>GQDMVSPPPPIADEPLTVNTGIYLIACYSLDDKAETFKVNAFLSLSWKDRRLAFDPVRSGVRVKTYEPEAIWIPEIRFVNVENARDADVVDISVSPDGTVQYLERFSARVLSPLDFRRYPFDSQTLHIYLIVRSVDTRNIVLAVDLEKVGKNDDVFLTGWDIESFTAVVKPANFALEDRLESKLDYQLRISRQYFSYIPNIILPMLFILFISWTAFWSTSYEANVTLVVSTLIAHIAFNILVETNLPKTPYMTYTGAIIFMIYLFYFVAVIEVTVQHYLKVESQPARAASITRASRIAFPVVFLLANIILAFLFFGF[5x]

At present, the best structurally characterized pLGIC is the G. violaceus ligand-gated ion channel (GLIC), of prokaryotic origin. Each subunit consists of an extracellular domain (ECD), predominantly in a β-sandwich fold, and a transmembrane domain (TMD) composed of four helices, labeled M1–M4. However, the GLIC is a pH-gated channel, activated by lowering the pH, with a maximal activation at pH 4 and a pH50 around 5. We instead found that proton activation is a complex multiple loci mechanism, with the key contribution stemming from the coupling interface between the extracellular and transmembrane domain, with E35 acting as a key proton-sensing residue.

In contrast to the nonsignificant individual mutations, E26, which is found interacting with the bottom of the β4-β5 loop of the principal (+) face, shows a robust decrease of the pH50 when mutated to both Q and A. A combination of E26Q with mutations of vestibular-facing residues that tend to decrease the pH50 produces an obvious decrease in pH50. A structural analysis was performed on E26Q, E26A, E35Q, E35A, E67A, E75A, E82Q, E82A, D86A, D88N, D88A, H127N, E181A, and H277Q mutants, by solving their structure at pH 4. The key mutants at E26, D86, and D88 were solved at pH 4, each showing a structure similar to that of the Wt. All structures were in the apparently open conformation. E26 clearly is an important residue in GLIC function, but other techniques are required to elucidate its mechanistic role. The report identified E26 and E177 to have loss-of-function effects when mutated. E26 indeed results in a loss-of-function effect, whereas E177 seems to have no effect.> MKTLVHVASVEKGRSYEDFQKVYNAIALKLREDDEYDNYIGYGPVLVRLAWHISGTWDKHDNTGGSYGGTYRFKKEFNDPSNAGLQNGFKFLEPIHKEFPWISSGDLFSLGGVTAVQEMQGPKIPWRCGRVDTPEDTTPDNGRLPDADKDAGYVRTFFQRLNMNDREVVALMGAHALGKTHLKNSGYEGPGG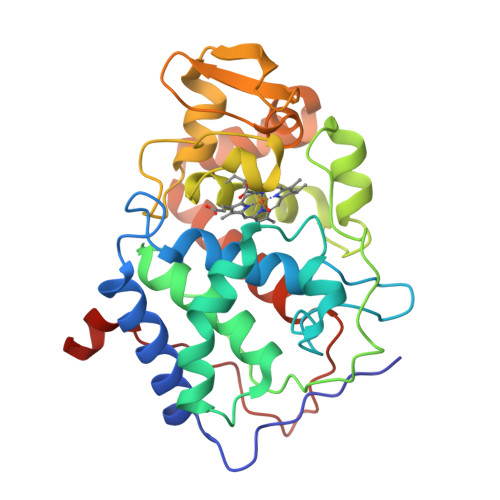AANNVFTNEFYLNLLNEDWKLEKNDANNEQWDSKSGYMMLPTNYSLIQDPKYLSIVKEYANDQDKFFKDFSKAFEKLLENGITFPKDAPSPFIFKTLEEQGL> SNANNARQARVAQSYENSYEVDSPAVRDSVLEAARQYNTSVVGFPILDPWLNRASKNSGPYLDYLQQLNPQRAERPVIASISIPTIDAHLPIYHGTDTATL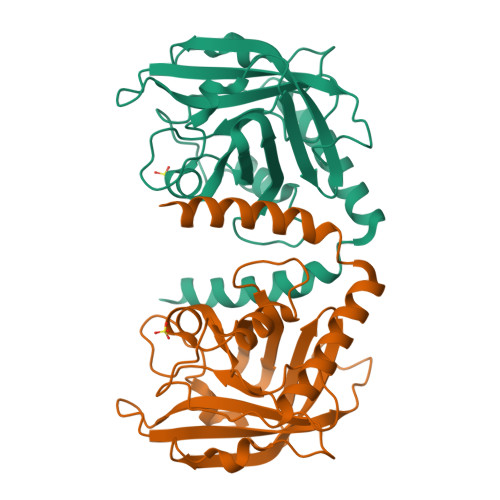EHGLGHLYGSALPVGGTGTHPVITGHSGLANATLFDNLEDVKEHDPIYITVQGETLKYEVDAINVVLPEDTKLLAPDPNKDQITLITCTPYAVNSHRLLVRAHRVDLDPNDPNL> MDTSNLMEQILSSDNLNRAYLQVVRNKGAEGVDGMKYTELKEHLAKNGETIKGQLRTRKYKPQPARRVE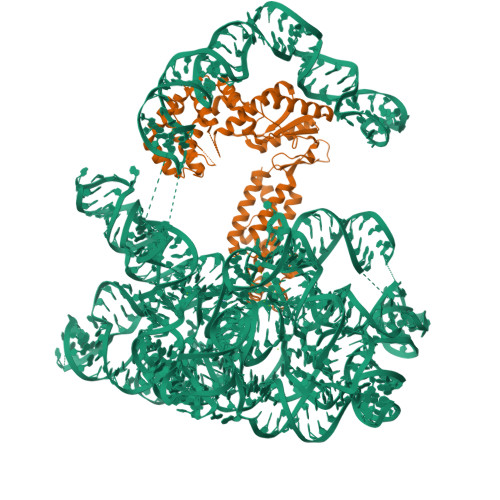IPKPDGGVRNLGVPTVTDRFIQQAIAQVLTPIYEEQFHDHSYGFRPNRCAQQAILTALNIMNDGNDWIVDIDLEKFFDTVNHDKLMTLIGRTIKDGDVISIVRKYLVSGIMIDDEYEDSIVGTPQGGNLSPLLANIMLNELDKEMEKRGLNFVRYADDCIIMVGSEMSANRVMRNISRFIEEKLGLKVNMTKSKVDRPSGLKYLGFGFYFDPRAHQFKAKPHAKSVAKFKKRMKELTCRSWGVSNSYKVEKLNQLIRGWINYFKIGSMKTLCKELDSRIRYRLRMCIWKQWKTPQNQEKNLVKLGIDRNTARRVAYTGKRIAYVCNKGAVNVAISNKRLASFGLISMLDYYIEKCVTC tetradecyl 4-O-alpha-D-glucopyranosyl-beta-D-glucopyranoside 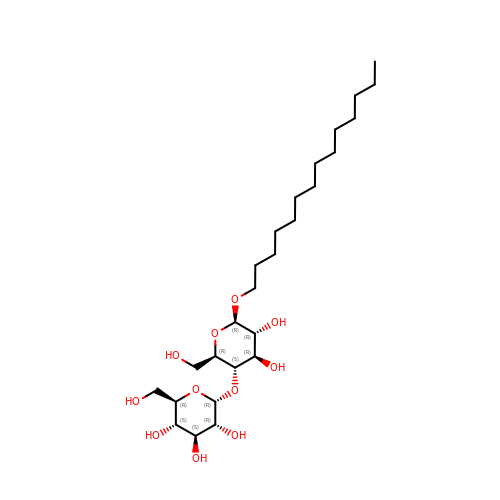| C26 H50 O11 | UKPROSIGWJBJGA-IWODYCRQSA-N>[2x]CELDRDPEGKDFQQPYTSFVQTKQNRDGLYALLRNTENPRMHFYQELQSDMYCTTITDGNSLAPFVNWDLGILNDHGRADEDEVSGIAGYYFVYNRLNQQANAFVNNTEAALQNQVYKNSTEIANAKSFLAEGKVLQALAIWRLMDRFSFHESVTEVNSGAKDLGVILLKEYNPGYIGPRATKAQCYDYILSRLSEAIEVLPENRESVLYVSRDYAYALRARIYLALGEYGKAAADAKMVVDKYPLIGAADASEFENIYRSDANNPEIIFRGFASATLGSFTATTLNGAAPAGKDIKYNPSAVPFQWVVDLYENEDFRKSVYIAKVVKKDKGYLVNKFLEDKAYRDVQDKPNLKVGARYFSVAEVYLILVESALQTGDTPTAEKYLKALSKARGAEVSVVNMEALQAERTRELIGEGSRLRDMVRWSIPNNHDAFETQPGLEGFANTTPLKAQAPVGFYAYTWEFPQRDRQTNPQLIKNWPI;> LSTVSGSVAKVSSEKLAEKPVANIMDALQGQVAGMQVMTTSGDPTAVASVEIHGTGSLGASSAPLYIVDGMQTSLDVVATMNPNDFESMSVLKDASATSIYGARAANGVVFIQTKKGKMSERGRITFNASYGISQILNTKPLDNMMTGDELLDFQVKAGFWGNNQTVQKVKDMILAGAEDLYGNYDSLKDEYGKTLFPVDFNHDADWLKALFKTAPTSQGDISFSGGSQGTSYYASIGYFDQEGMAREPANFKRYSGRLNFESRINEWLKVGANLS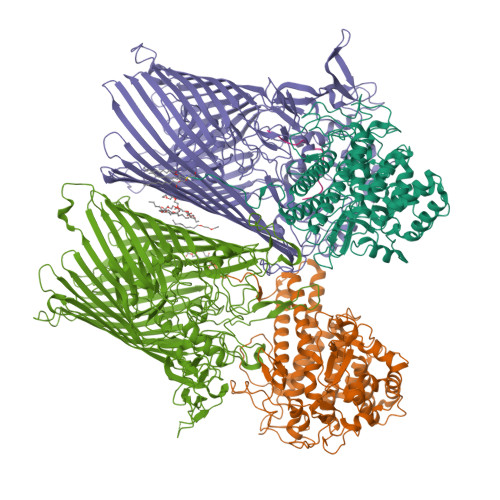GAIANRRSADYFGKYYMGSGTFGVLTMPRYYNPFDVNGDLADVYYMYGATRPSMTEPYFAKMRPFSSESHQANVNGFAQITPIKGLTLKAQAGVDITNTRTSSKRMPNNPYDSTPLGERRERAYRDVSKSFTNTAEYKFSIDEKHDLTALMGHEYIEYEGDVIGASSKGFESDKLMLLSQGKTGNSLSLPEHRVAEYAYLSFFSRFNYGFDKWMYIDFSVRNDQSSRFGSNNRSAWFYSVGGMFDIYNKFIQESNWLSDLRLKMSYGTTGNSEIGNYNHQALVTVNNYTEDAMGLSISTAGNPDLSWEKQSQFNFGLAAGAFNNRLSAEVDFYVRTTNDMLIDVPMPYISGFFSQYQNVGSMKNTGVDLSLKGTIYQNKDWNVYASANFNYNRQEITKLFFGLNKYMLPNTGTIWEIGYPNSFYMAEYAGIDKKTGKQLWYVPGQVDADGNKVTTSQYSADLETRIDKSVTPPITGGFSLGASWKGLSLDADFAYIVGKWMINNDRYFTENGGGLMQLNKDKMLLNAWTEDNKETDVPKLGQSPQFDTHLLENASFLRLKNLKLTYVLPNSLFAGQNVIGGARVYLMARNLLTVTKYKGFDPEAGGNVGKNQYPNSKQYVAGIQLSF;> SGATTATTTTSNS;> QVVVLGYGTGQKLSTVSGSVAKVSSEKLAEKPVANIMDALQGQVAGMQVMTTSGDPTAVASVEIHGTGSLGASSAPLYIVDGMQTSLDVVATMNPNDFESMSVLKDASATSIYGARAANGVVFIQTKKGKMSERGRITFNASYGISQILNTKPLDNMMTGDELLDFQVKAGFWGNNQTVQKVKDMILAGAEDLYGNYDSLKDEYGKTLFPVDFNHDADWLKALFKTAPTSQGDISFSGGSQGTSYYASIGYFDQEGMAREPANFKRYSGRLNFESRINEWLKVGANLSGAIANRRSADYFGKYYMGSGTFGVLTMPRYYNPFDVNGDLADVYYMYGATRPSMTEPYFAKMRPFSSESHQANVNGFAQITPIKGLTLKAQAGVDITNTRTSSKRMPNNPYDSTPLGERRERAYRDVSKSFTNTAEYKFSIDEKHDLTALMGHEYIEYEGDVIGASSKGFESDKLMLLSQGKTGNSLSLPEHRVAEYAYLSFFSRFNYGFDKWMYIDFSVRNDQSSRFGSNNRSAWFYSVGGMFDIYNKFIQESNWLSDLRLKMSYGTTGNSEIGNYNHQALVTVNNYTEDAMGLSISTAGNPDLSWEKQSQFNFGLAAGAFNNRLSAEVDFYVRTTNDMLIDVPMPYISGFFSQYQNVGSMKNTGVDLSLKGTIYQNKDWNVYASANFNYNRQEITKLFFGLNKYMLPNTGTIWEIGYPNSFYMAEYAGIDKKTGKQLWYVPGQVDADGNKVTTSQYSADLETRIDKSVTPPITGGFSLGASWKGLSLDADFAYIVGKWMINNDRYFTENGGGLMQLNKDKMLLNAWTEDNKETDVPKLGQSPQFDTHLLENASFLRLKNLKLTYVLPNSLFAGQNVIGGARVYLMARNLLTVTKYKGFDPEAGGNVGKNQYPNSKQYVAGIQLSF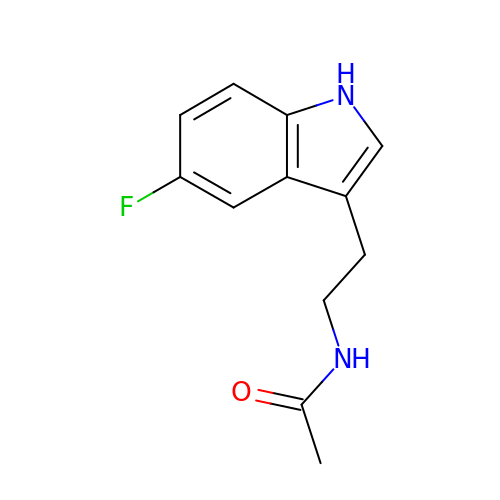~{N}-[2-(5-fluoranyl-1~{H}-indol-3-yl)ethyl]ethanamide | C12 H13 F N2 O | UDLASALUJLTGJV-UHFFFAOYSA-N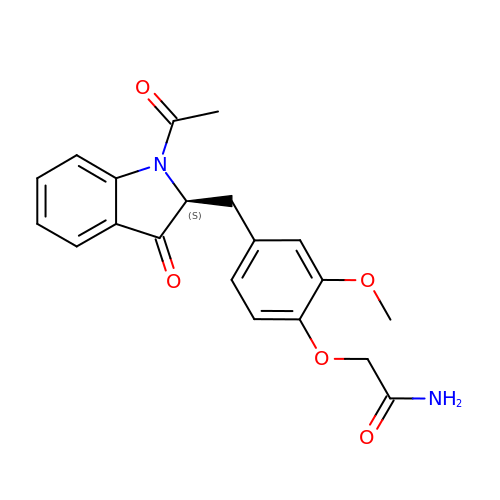2-[4-[[(2S)-1-ethanoyl-3-oxidanylidene-2H-indol-2-yl]methyl]-2-methoxy-phenoxy]ethanamide | C20 H20 N2 O5 | DUXGCVPXJWCVOO-INIZCTEOSA-N> IVGGTASVRGEWPWQVTLHTTSPTQRHLCGGSIIGNQWILTAAHCFYGVESPKILRVYSGILNQSEIKEDTSFFGVQEIIIHDQYKMAESGYDIALLKLETTVNYTDSQRPISLPSKGERNVIYTDCWVTGWGYRKLRDKIQNTLQKAKIPLVTNEECQKRYRGHKITHKMICAGYREGGKDACKGDSGGPLSCKHNEVWHLVGITSWGEGCA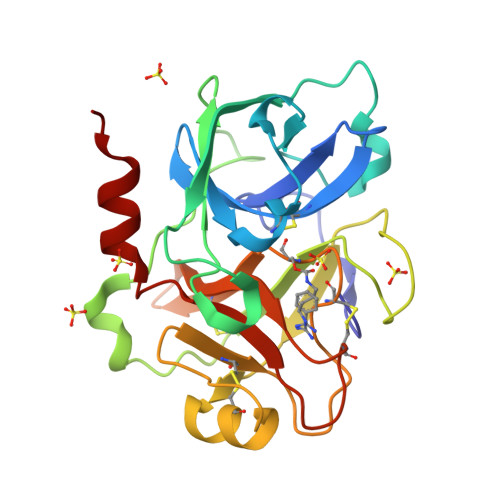QRERPGVYTNVVEYVDWILEKTQAV> DAASDLKSRLDKVSSFHASFTQKVTDGSGAAVQEGQGDLWVKRPNLFNWHMTQPDESILVSDGKTLWFYNPFVEQ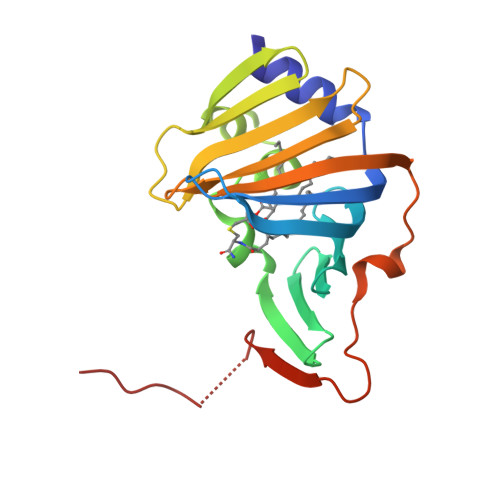ATATWLKDATGNTPFMLIARNQSSDWQQYNIKQNGDDFVLTPKASNGNLKQFTINVGRDGTIHQFSAVEQDDQRSSYQLKSQQNGAVDAAKFTFTPPQGVTVDDQRKGSWSHPQFEK> IVGGYTCEENSLPYQVSL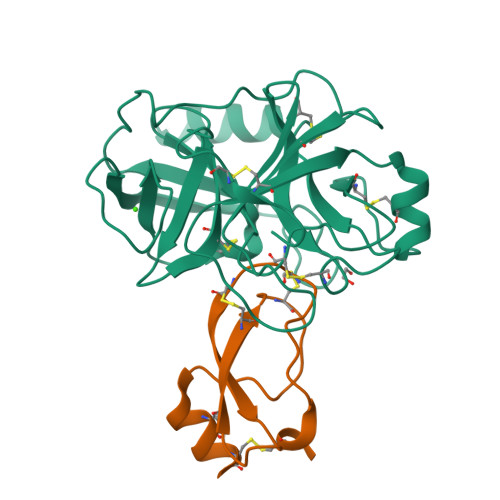NSGSHFCGGSLISEQWVVSAAHCYKTRIQVRLGEHNIKVLEGNEQFINAAKIIRHPKYNRDTLDNDIMLIKLSSPAVINARVSTISLPTAPPAAGTECLISGWGNTLSFGADYPDELKCLDAPVLTQAECKASYPGKITNSMFCVGFLEGGKDSCQRDAGGPVVCNGQLQGVVSWGHGCAWKNRPGVYTKVYNYVDWIKDTIAANS;> YVDYKDDDDKEFEVCSEQAETGPCRACFSRWYFDVTEGKCAPFCYGGCGGNRNNFDTEEYCMAVCGSAIPRHHHHHHAAA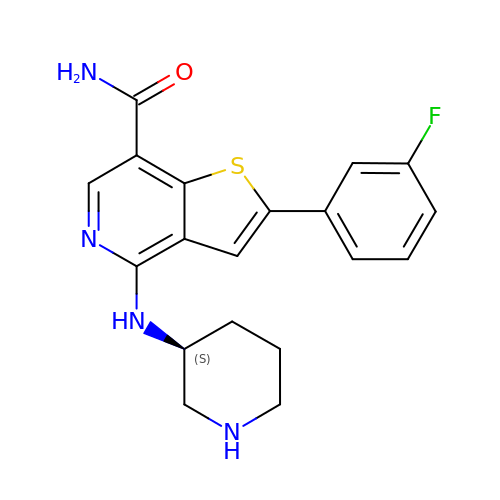2-(3-fluorophenyl)-4-[[(3~{S})-piperidin-3-yl]amino]thieno[3,2-c]pyridine-7-carboxamide | C19 H19 F N4 O S | YTDCGNUVVIXLSO-ZDUSSCGKSA-N> GDKLHEIKQELKDLFSHLPYKINKVEVSLYEPGVLLIDIDGEDSALLIGEKGYRYKALSYLLFNWIHPTYGYSIRLEISTFLQNQEKVMDTQLQSVIMTVHEVGKGQMKAPDGVLTYIALKKLRKAFPNKYVSIKTNLN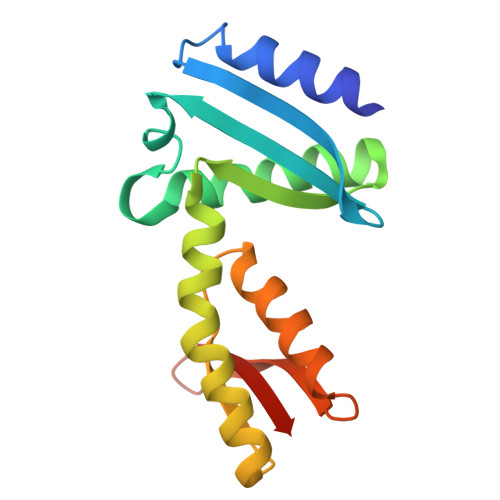DEKYIVINDFNNE> AHMQHSKSSVHAELRELPESTANLIENSHADDVFSPNMVERLWVLAKSTRDSAQMSDSIISSLSDVLVLSPLEVLASWYAADLLDALLMESLSRKVEISEIEEIISLCPKNSSIIRHALLAKLVLFPENTADSLNEVLAAYKNTLDLCSQDKRKQSSVLKINLSKLFTLHSCLSLALQRLGYGDVSKRMYQEIFVPDSDADITPLSFIISWTALNTFAPICTSPKENDVVEKMAMY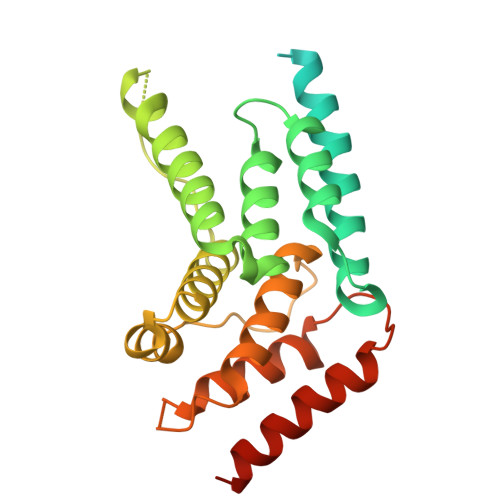VRTAIGTLKIQDLKLSRKLINSCIDIGSRLQEDLGY> GCCACCCUG;> CAGGGUCG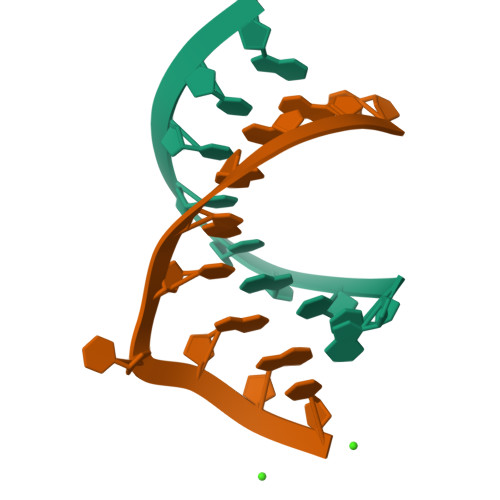GC>[2x]MSNSAETDVLIVGAGPAGAMSATLLASLGIRSLMINRWRSTSPGPRSHIINQRTMEILRDIGLEESAKSLAVPKEYMGEHVYATSLAGEEFGRIPAWASHPQAHAEHELASPSRYCDLPQLYFEPMVVS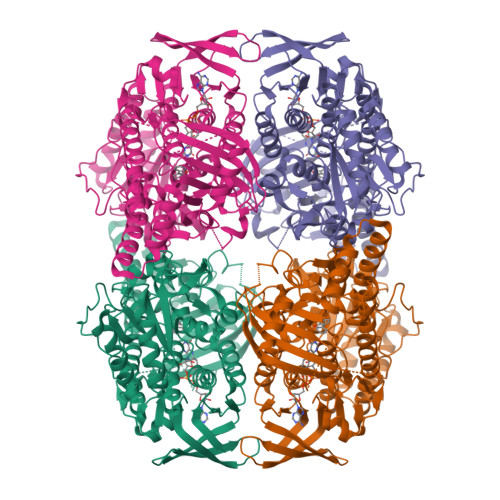EAALRGADVRFLTEYLGHVEDQDGVTARLLDHVSGAEYEVRAKYIIGADGAHSLVAQNAGLPFEGQMGIGDSGSINIEFSADLSSLCEHRKGDMYWMFRAGSGINGVGVAALRMIRPWNKWICVWGYEKSKGTPEITKEEAKKIIHEIIGTDEIPVEVGPISTWTINQQYAVRNTSGRVFCMGDAVHRHTPMGGLGLNTSVQDAYNLAWKLALVLKGTAAPTLLDSYDAERSPVAKQIVERAFKSLSTFPPVFEALSLPPAPTESEMAEALVRLKDASEEGAKRRAALRKAMDATIIGLGGGHGVELNQRYVSRAVFPDGTPDPGFVRDQEFFYQASTRPGAHLPHVWLTENQRRISTLDLCGKGRFTLLTGLSGAAWKHEAEQVSQSLGIELKVCVIGPGQEFVDTYGEYAKISEIGESGALLVRPDMFIAFRAKDASREGLEQLNVAVKSILGRA>MKVGSQVIINTSHMKGMKGAEATVTGAYDTTAYVVSYTPTNGGQRVDHHKWVIQEEIKDAGDKTL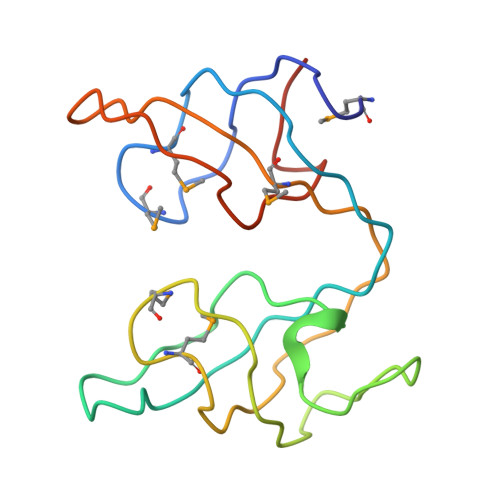QPGDQVILEASHMKGMKGATAEIDSAEKTTVYMVDYTSTTSGEKVKNHKWVTEDELLEHHHHHH[3x]N-(3-carbamoyl-5,5,7,7-tetramethyl-4,7-dihydro-5H-thieno[2,3-c]pyran-2-yl)-1H-pyrazole-3-carboxamide | 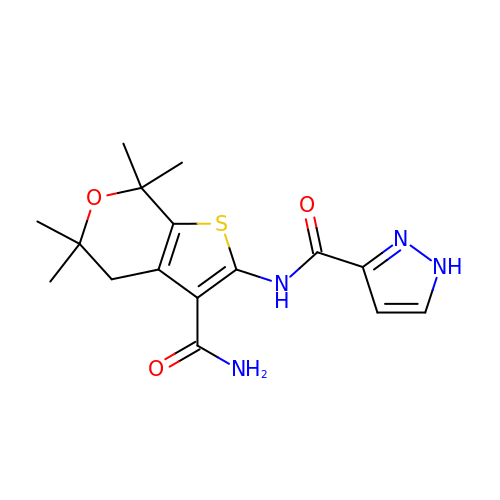C16 H20 N4 O3 S | GHTGYZMBQPXTCQ-UHFFFAOYSA-N>MKQLATPFQEY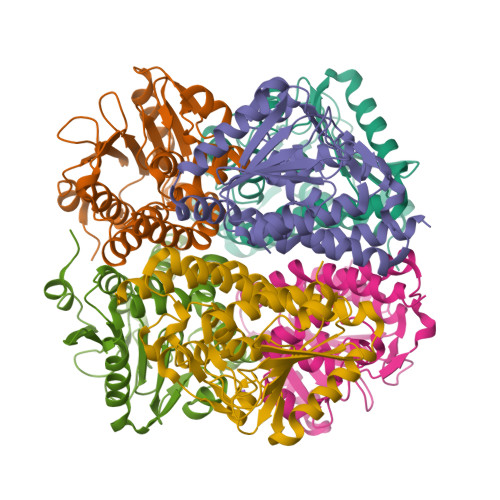SQKYENIRLERDGGVLLVTVHTEGKSLVWTSTAHDELAYCFHDIACDRENKVVILTGTGPSFCNEIDFTSFNLGTPHDWDEIIFEGQRLLNNLLSIEVPVIAAVNGPVTNHPEIPVMSDIVLAAESATFQDGPHFPSGIVPGDGAHVVWPHVLGSNRGRYFLLTGQELDARTALDYGAVNEVLSEQELLPRAWELARGIAEKPLLARRYARKVLTRQLRRVMEADLSLGLAHEALAAIDLGMESEQ[6x]>[2x]RPSDPGVVSYAVMPKGSVSNIVGAPIRWESEFTAPFQAFSVDNPVCNNWADIGLPEVFNDPDLASFGGATAQTAAGDATHLVKQAVGVFATVDAADRAY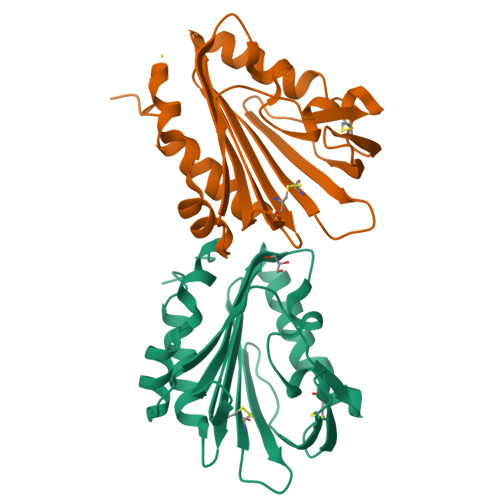HRVVDRTVGCAGQTTAMHLDNFHTEVWTFTGGPAGPADADWVKQEAGTDRRCFNTTRKRENVLLQAKVCQSGNGGPAVNVLAGAMQNTLGQLEHHHHHH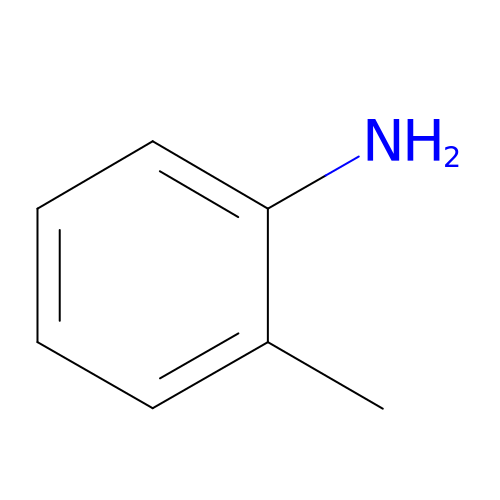2-methylaniline | C7 H9 N | RNVCVTLRINQCPJ-UHFFFAOYSA-N Acid ceramidase (aCDase; ASAH1) is the best studied member of the family and is prominent for its involvement in Farber disease (FD), a genetic disorder in humans. aCDase is ubiquitously expressed and found in the lysosome where it normally regulates sphingolipid metabolism through intralysosomal membrane turnover. Similar to other Ntn-hydrolases, aCDase is synthesized as an inactive proenzyme that requires proteolysis for activation. The α-subunit consists of a globular helical domain formed by five α-helices preceded by a 36-residue linker region, whereas the β-subunit contains two central anti-parallel β-sheets flanked on either side by a total of six α-helices.

A third structure is of the heterodimeric activated state from human, which was allowed to fully autocleave before crystallization. The overall structure of the enzyme does not change significantly after autocleavage (1.1 Å r.m.s.d.), but there are conformational changes at the junction between the α- and β-subunits. First, residues 141 and 142 at the C terminus of the newly created α-subunit become disordered. Second, the last turn of the C-terminal helix-α5 of the α-subunit (residues 135 to 140) bends “away” from the enzyme by roughly 60°. The channel is composed of a constellation of mainly hydrophobic residues, presumably to accommodate the ceramide acyl chains, while directing the scissile amide bond towards the active site. In addition to uncovering the substrate-binding site upon autocleavage, the concomitant conformational change to the α-β junction causes strand-β3 containing Cys 143 to shift. This moves Cys 143 away from Arg 159 breaking their putative hydrogen bond, suggesting that for substrate cleavage Arg 159 may not act as the general base. The tightly bound water, W1, from the proenzyme is no longer present, as it would clash with Cys 143 and presumably is no longer required because the active site is now accessible to the outside environment. The active structure of human-aCDase allowed us to map these mutations to rationalize their potential effects.

>DRHHHHHHKLQHAPPWTEDCRKSTYPPSGPTYRGAVPWYTINLDLPPYKRWHELMLDKAPMLKVIVNSLKNMINTFVPSGKVMQVVDEKLPGLLGNFPGPFEEEMKGIAAVTDIPLGEIISFNIFYELF[2x];>[2x]TICTSIVAEDKKGHLIHGRNMDFGVFLGWNINNDTWVITEQLKPLTVNLDFQRNNKTVFKASSFAGYVGMLTGFKPGLFSLTLNERFSINGGYLGILEWILGKKDAMWIGFLTRTVLENSTSYEEAKNLLTKTKILAPAYFILGGNQSGEGCVITRDRKESLDVYELDAKQGRWYVVQTNYDRWKHPFFLDDRRTPAKMCLNRTSQENISFETMYDVLSTKPVLNKLTVYTTLIDVTKGQFETYLRDCPDPCIGW>[3x]MGRPRKDSRLMPVSLSVQSPAALTAEKEAMCLSAPALALKLPIPS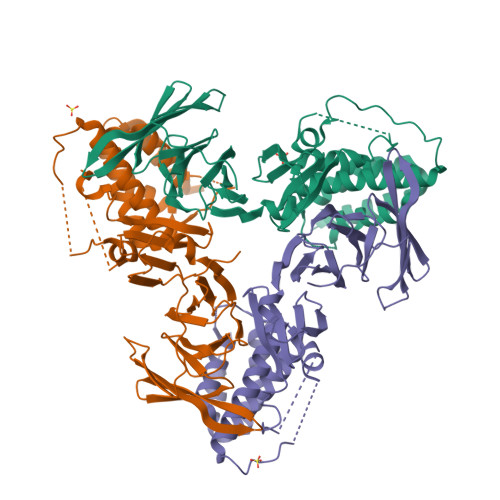PQRAFTLQVSSDPSMYIEVENEVTVVGGVKLSRLKCNREGKEWETVLTSRILTAAGSCDVVCVACEKRMLSVFSTCGRRLLSPILLPSPISTLHCTGSYVMALTAAATLSVWDVHRQVVVVKEESLHSILAGSDMTVSQILLTQHGIPVMNLSDGKAYCFNPSLSTWNLVSDKQDSLAQCADFRSSLPSQDAMLCSGPLAIIQGRTSNSGRQAARLFSVPHVVQQETTLAYLENQVAAALTLQSSHEYRHWLLVYARYLVNEGFEYRLREICKDLLGPVHYSTGSQWESTVVGLRKRELLKELLPVIGQNLRFQRLFTECQEQLDILRDKLEGSS>[4x]MSLSKLDIPLSIMQKSVVIRPGGRQEMDEHVAIETPYAIALNDRVIGSSMVLPVDLEEFGAGFLFGQGYIKKAEEIREILVCPQGRISVYADVENEEPREVIITSGCGGTGKIPKEMLEGEFAPLADYCLPFAEIKSFIREALHSSPLGPQTHCVHGCGLWNNGRLQVYHEDVGRHNAVDKVLGSILLGRASNNSAVYTTGRLTSDMVLKCARIGIPIIMSRT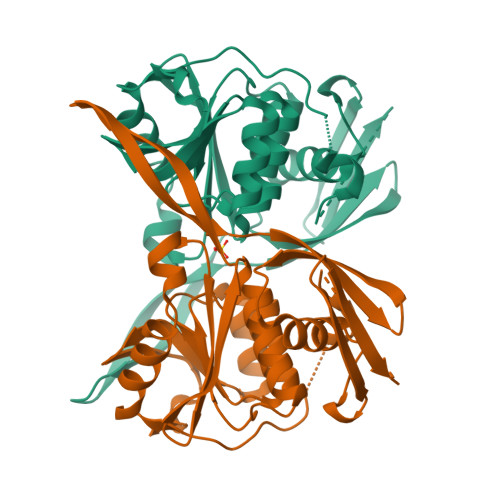SPSSLGLALAKRSGATLVAYSRPERINVFNAPERILTEGHHHHHH>[2x]GAMGHAPAPSESQRLVRRVVIAGGGTAGWMAAAALSKLLGRQLQITLVESDEIGTVGVGEATIPSLVTFHRLLEIDEAQFMAATQATFKVGIAFEHWRDVDRHYIHSFGHTGTDHWSAGFQHFWLKAHARGVARDFGDYCLELRAAQEGRFAHLPNGGMNYAYHLDAGLYARFLRRFSEGFGVQRIEGRIGSVQTDAHSGDIAALVLDDGTRIEGDLFLDCTGFRALLIGQTLGVGSEDWSRWLFADSALAVQTESVGAPVTFTRARADRAGWMWRIPLQHRVGNGIVYSSRYTDQDSAAQVLEHNLQGRALTTPRALRFTPNQRHR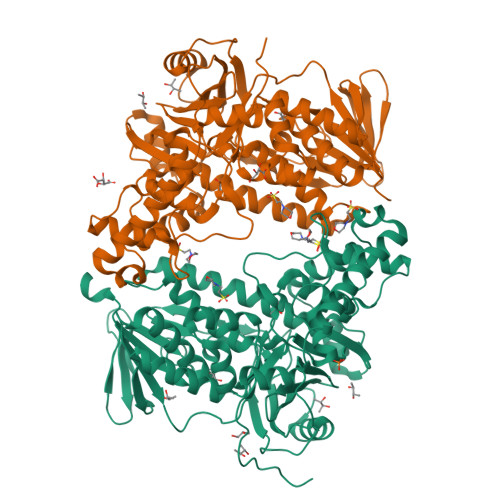VWEKNCVALGLASGFLEPIESTNIHLIQRGIVRLLQTFPQVIDPVDIAEYNRQAAEEIAHIRDFVILHYHATDRRDTAFWRDCASMEIPDSLRHRMELFRQSGRVFHQGNELFAENSWIQVMLGQGIVPRHHHPVADLMGDAELSQFLEGIRQRVEATLARLPPHAEFLRRYCPAPAPPAPMPQPAPGTPLAAPAA> MRLLYLHADRFEYKTVKPALKNPPDPPGEASFGEALVVFTTVEDGDGPQTVMYAASDIASH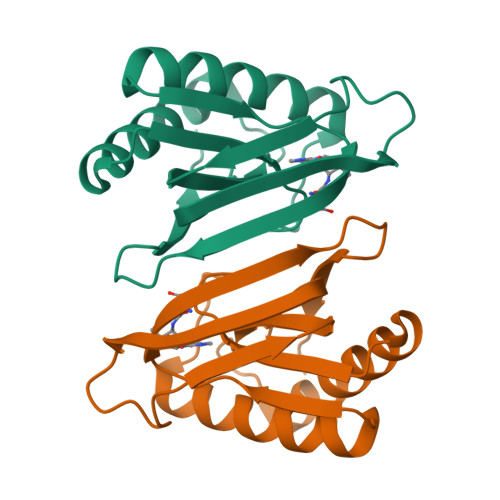SSRLKVTTVILYPYAHLSSRLAKPMAAHKRLIELEGALRTKFPGHVHRAPFGWAKSFSIACKGHPLAELSRSFTE>[2x]MIVDQFEEVLMKTSQLFPLPTATQSAQPTHVAPVPTVLPDTPIYETVGDSGSKTLWVVFVLMLIASAAFTALSWKIPVNRRLYHVITTIITLTAALSYFAMATGHGVALNKIVIRTQHDHVPDTYETVYRQVYYARYIDWAITTPLLLLDLGLLAGMSGAHIFMAIVADLIMVLTGLFAAFGSEGTPQKWGWYTIACIAYIFVVWHLVLNGGANARVKGEKLRSFFVAIGAYTLILWTAYPIVWGLADGARKIGVDGEIIAYAVLDVLAKGVFGAWLLVTHANLRESDVELNGFWANGLNREGAIRIGEDDGAGTHHHHHHHHH

Type 1 rhodopsins are heptahelical transmembrane (7TM) proteins that covalently bind the retinal chromophore and use the energy of light to perform different biological functions, such as ion pumping, ion channeling, sensoring, and kinase activity. To fill this gap in the current understanding of the proton pumps and to gain insight into the evolution of rhodopsins using a structure-based approach, we performed a structural and functional analysis of the light-driven proton pump LR (Mac) from the pathogenic fungus Leptosphaeria maculans. The first high-resolution structure of fungi rhodopsin and its functional properties reveal the striking similarity of its membrane part to archaeal but not to bacterial rhodopsins. We compare to our knowledge all available structures and sequences of outward light-driven proton pumps and show that eukaryotic and archaeal proton pumps, most likely, share a common ancestor.

Here we present the first high-resolution, at 2.2 Å, crystal structure of a light-driven H+ pump from fungi and elucidate the functional role of the N-terminal region. The crystals belong to the P21 space group and comprise two protomers in an asymmetric unit. LR (residues 42–286), all-trans-retinal (ATR), 19 lipid molecules, and 65 water molecules inside the protein are clearly resolved in the electron-density map, whereas the N- and C-terminal domains lack resolution for 41 and 31 residues, respectively. The LR bundle consists of seven transmembrane helices-TM1–TM7, connected by three intracellular (ICL 1–3) and three extracellular (ECL 1–3) loops, with retinal chromophore covalently attached to the K270 on the TM7. The interior portions of LR and HsBR are virtually identical structurally, and the only major difference is observed at the extracellular sides of these rhodopsins. In the LR structure, the retinal chromophore is fixed in an all-trans conformation. The protonated retinal Schiff base (RSB) points toward the extracellular side and donates a hydrogen bond to the w8 molecule. This arrangement is stabilized by the RSB counterions, D266 and D139, which are counterparts to D212 and D85 in HsBR. Consistent with the prediction, the LR crystal structure contained 8 residues from the N-terminal region (residues 42–49), that aligned with ECL1 and belonged to a 3-stranded antiparallel β-sheet. This N-terminal β-strand strongly interacts with the ECL1 loop and is directly involved in its stabilization through at least 7 hydrogen bonds.1H-IMIDAZOL-2-YLMETHANOL | C4 H6 N2 O | 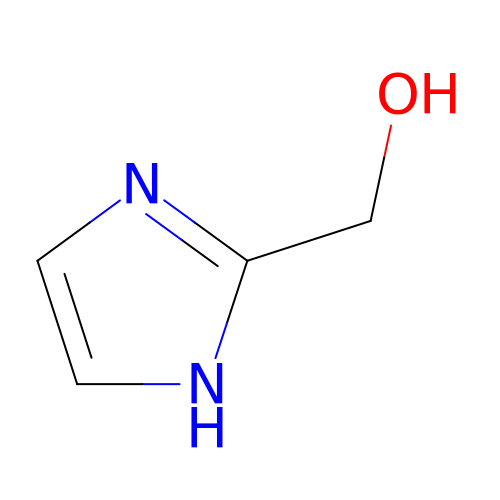ZOMATQMEHRJKLO-UHFFFAOYSA-N> MEDKGKTFFGQPLGLSTLFMTEMWERFSYYGMRAILLYYMWFLISTGDLHITRATAASIMAIYASMVYLSGTIGGFVADRIIGARPAVFWGGVLIMLGHIVLALPFGASALFGSIILIIIGTGFLKPNVSTLVGTLYDEHDRRRDAGFSIFVFGINLGAFIAPLIVGAAQEAAGYHVAFSLAAIGMFIGLLVYYFGGKKTLDPHYLRPTDPLAPEEVKPLLVKVSLAVAGFIAIIVVMNLVGWNSLPAYINLLTIVAIAIPVFYFAWMISSVKVTSTEHLRVVSYIPLFIAAVLFWAIEEQGSVVLATFAAERVDSSWFPVSWFQSLNPLFIMLYTPFFAWLWTAWKKNQPSSPTKFAVGLMFAGLSFLLMAIPGALYGTSGKVSPLWLVGSWALVILGEMLISPVGLSVTTKLAPKAFNSQMMSMWFLSSSVGSALNAQLVTLYNAKSEVAYFSYFGLGSVVLGIVLVFLSKRIQGLMQGVEGSENLYFQ;> AAA

To address this question, we determined high-resolution crystal structures of a bacterial homologue to the mammalian PepT1 protein from Streptococcus thermophilus, PepTSt in complex with physiologically relevant di- and tripeptides in addition to a peptide-free apo form. The POT/PTR family contains a number of conserved sequence motifs and a conserved architecture consisting of 12 or 14 transmembrane α-helices arranged into N (H1–6)- and C-terminal (H7–12) bundles 3,10–12. A centrally located peptide-binding site is highly conserved between prokaryote and eukaryote members, with both operating via similar transport mechanisms. Conserved pairs of salt bridge interactions coordinate structural rearrangements that lead to the vectorial co-transport of peptides and protons across the membrane 3,11.

A new crystal structure in complex with the tripeptide l-Ala-l-Ala-l-Ala (tri-Ala), which was the only tested tripeptide to inhibit di-Ala transport, was obtained and refined to a final resolution of 2.5 Å. Careful analyses of the electron density maps, including the calculation of simulated annealing OMIT maps and averaged kick maps 18, clearly showed the tri-Ala peptide sitting in a vertical orientation. The data, however, do not allow us to establish how the peptide is orientated in the binding site, with its C-terminus facing towards the cytoplasmic or periplasmic space. This ambiguity arises due to ill-defined electron density that likely reflects low occupancy of the peptide in the binding site. c PepTSt tri-Ala complex was deposited with the carboxy terminus of the tripeptide oriented towards the extracellular side of the membrane. The tripeptide sits in an elongated cavity formed by H1 (Tyr30), H5 (Asn156), H7 (Glu299, 300) and H8 (Gln325, Asn328) and above the alanine side chain observed in the Ala-Phe complex. Compared to the Ala-Phe complex, tri-Ala makes far fewer interactions with the protein. Another noticeable difference is the presence of a third smaller cavity (pocket 3) that opens up opposite the third side chain in the tri-Ala peptide as a result of the less compact structure adopted by PepTSt in the tri-Ala complex compared to the Ala-Phe complex. The nitrogen of the C-terminal peptide bond in tri-Ala peptide interacts with the side chain of Tyr30. By comparison, the same Asn156Ala variant had no effect on tri-Ala competition, consistent with the complex structure where Asn156 does not interact with the tri-Ala peptide.> MHHHHHHSSGRENLYFQGMTVREKTRLEKFRQLLSSQNTDLDELRKCSWPGVPREVRPITWRLLSGYLPANT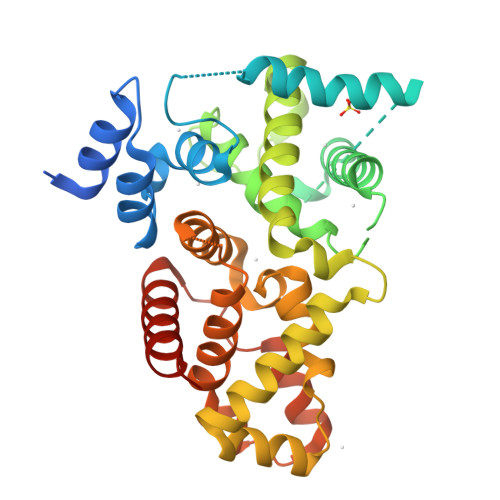ERRKLTLQRKREEYFGFIEQYYDSRNEEHHQDTYRQIHIDIPRTNPLIPLFQQPLVQEIFERILFIWAIRHPASGYVQGINDLVTPFFVVFLSEYVEEDVENFDVTNLSQDMLRSIEADSFWCMSKLLDGIQDNYTFAQPGIQKKVKALEELVSRIDEQVHNHFRRYEVEYLQFAFRWMNNLLMRELPLRCTIRLWDTYQSEPEGFSHFHLYVCAAFLIKWRKEILDEEDFQGLLMLLQNLPTIHWGNEEIGLLLAEAYRLKYMFADAPNHYRR>[2x]GPLGSMADAAPQLGKRKRELDVEEAHAASTEEKEAGVGNGTCAPVRLPFSGFRLQKVLRESARDKIIFLHGKVNEASGDGDGEDAVVILEKTPFQVEQVAQLLTGSPELQLQFSNDIYSTYHLFPPRQLNDVKTTVVYPATEKHLQKYLRQDLRLIRETGDDYRNITLPHLESQSLSIQWV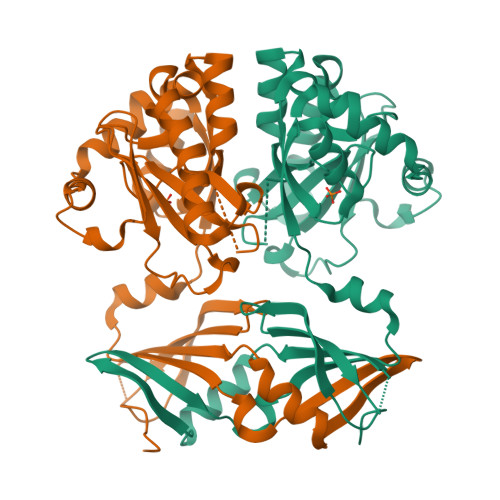YNILDKKAEADRIVFENPDPSDGFVLIPDMKWNQQQLDDLYLIAICHRRGIRSLRDLTPEHLPLLRNILHQGQEAILQRYRMKGDHLRVYLHYLPSYYHLHVHFTALGFEAPGSGVERAHLLAEVIENLECDPRHYQQRTMTFALRADDPLLKLLQEAQQS> MNHLGKTEVF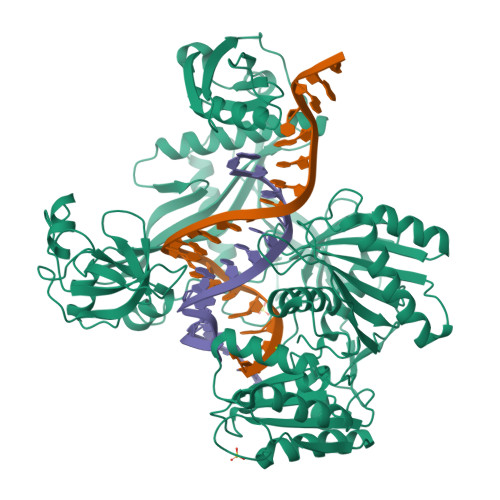LNRFALRPLNPEELRPWRLEVVLDPPPGREEVYPLLAQVARRAGGVTVRMGDGLASWSPPEVLVLEGTLARMGQTYAYRLYPKGRRPLDPKDPGERSVLSALARRLLQERLRRLEGVWVEGLAVYRREHARGPGWRVLGGAVLDLWVSDSGAFLLEVDPAYRILCEMSLEAWLAQGHPLPKRVRNAYDRRTWELLRLGEEDPKELPLPGGLSLLDYHASKGRLQGREGGRVAWVADPKDPRKPIPHLTGLLVPVLTLEDLHEEEGSLALSLPWEERRRRTREIASWIGRRLGLGTPEAVRAQAYRLSIPKLMGRRAVSKPADALRVGFYRAQETALALLRLDGAQGWPEFLRRALLRAFGASGASLRLHTLHAHPSQGLAFREALRKAKEEGVQAVLVLTPPMAWEDRNRLKALLLREGLPSQILNVPLREEERHRWENALLGLLAKAGLQVVALSGAYPAELAVGFDAGGRESFRFGGAACAVGGDGGHLLWTLPEAQAGERIPQEVVWDLLEETLWAFRRKAGRLPSRVLLLRNGRVPQDEFALALEALAREGIAYDLVSVRKSGGGRVYPVQGRLADGLYVPLEDKTFLLLTVHRDFRGTPRPLKLVHEAGDTPLEALAHQIFHLTRLYPASGFAFPRLPAPLHLADRLVKEVGRLGIRHLKEVDREKLFFV> MKAWVLKRLGGPLELVDLPEPEAEEGEVVLRVEAVGLNFADHLMRLGAYLTRLHPPFIPGMEVVGVVEGRRYAALVPQGGLAERVAVPKGALLPLPEGLSPEEAAAFPVSFLTAYLALKRAQARPGEKVLVQAAAGALGTAAVQVARAMGLRVLAAASRPEKLALPLALGAEEAATYAEVPERAKAWGGLD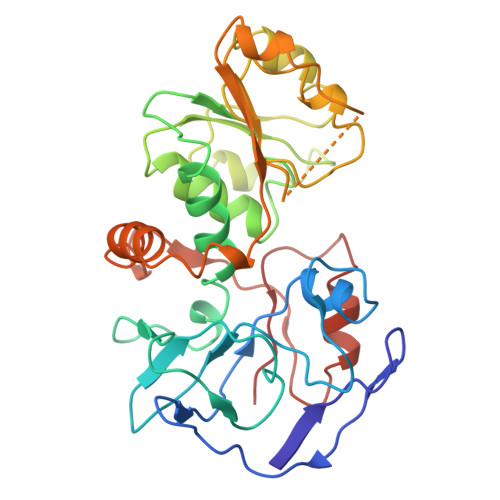LVLEVRGKEVEESLGLLAHGGRLVYIAPIPPLRLMRRNLAVLGFWLTPLLREGALVEEALGFLLPRLGRELRPVVGPVFPFAEAEAAFRALLDRGHTGKVVVRL>NPLFSPYKMGKFNLSHRVVLAPMTRCRALNNIPQAALGEYYEQRATAGGFLITEGTMISPTSAGFPHVPGIFTKEQVREWKKIVDVVHAKGAVIFCQLWHVGRASHEVYQPAGAAPISSTEKPISNRWRILMPDGTHGIYPKPRAIGTYEISQVVEDYRRSALNAIEAGFDGIEIHGAHGYLIDQFLKDGINDRTDEYGGSLANRCKFITQVVQAVVSAIGADRVGVRVSPAIDHLDAMDSNPLSLGLAVVERLNKIQLHSGSKLAYLHVTQPDYVAYGQTEAGRLGSEEEEARLMRTLRNAYQGTFICSGGYTRELGIEAVAQGDADLVSYGRLFISNPDLVMRIKLNAPLNKYNRKTFYTQDPVVGYTDYPFL[4x]

Jasmonates are phytohormones that are pivotal in mediating plant responses to various biotic and abiotic stresses and regulating plant growth. The first crystal structure of OPR3 from tomato (SlOPR3) showed that the enzyme crystallized as a self-inhibitory dimer in which the L6 loop, a critical loop involved in substrate recognition and coenzyme binding, from each protomer intrudes into the active site cavity of the other protomer. Based on these observations, it was postulated that the formation of the self-inhibitory homodimer represents a mechanism for regulating OPR3 activity and, thereby, jasmonic acid biosynthesis.

The self-inhibitory dimer of variant R283D differs from that of the wild type, as only loop L6 of one protomer intrudes into the active site of the other protomer, while the other loop only covers the active site entrance of the other protomer. As a result, the active site of only one protomer is entirely blocked while that of the other protomer is still accessible to at least small molecules, as evidenced by a bound MPD molecule above FMN. The folded hairpin-like structure of L6 that only covers the active site of the other protomer is stabilized by an intramolecular salt bridge network between E291, which usually lies above the flavin cofactor of the adjacent protomer, R294, and D243. In detail, D243 electrostatically holds back R294, which in turn prevents E291 from moving toward the active site of the adjacent protomer. Unfortunately, it is unclear from the structure how the amino acid substitution induces this semi-self-inhibitory dimer because D283 is not directly involved in stabilizing the folded L6 conformation. A comparison of the protomers in the R283D dimer shows that in protomer B, D283 forms a salt bridge with R343, like in the R283E dimer, whereas in protomer A, D283 is not involved in any interaction and thus free to move. We speculate that this freedom of movement translates to the whole loop L6, bringing D243, E291, and R294 together. D283 is located only 3.5 Å away from D243 and thus might push D243 toward R294 via electrostatic repulsion, indirectly supporting the salt bridge network that stabilizes the folded L6 conformation. However, in all cases, the strongest contribution to the dimer interface comes from the interactions of E291 with the catalytic residues H185 and H188, except for the semi-inhibitory R283D dimer in which E291 of one protomer interacts with R136 from the other protomer. Nevertheless, our crystallographic data show that substituting R283 for an oppositely charged residue generally affects L6 conformation and thus the dimerization process.>[3x]RRHKNKNPFHFNSKRFQTLFKNQYGHVRVLQRFNKRSQQLQNLRDYRILEFNSKPNTLLLPHHADADYLIVILNGTAILTLVNNDDRDSYNLQSGDALRVPAGTTYYVVNPDNDENLRMITLAIPVNKPGRFESFFLSSTQAQQSYLQGFSKNILEASYDTKFE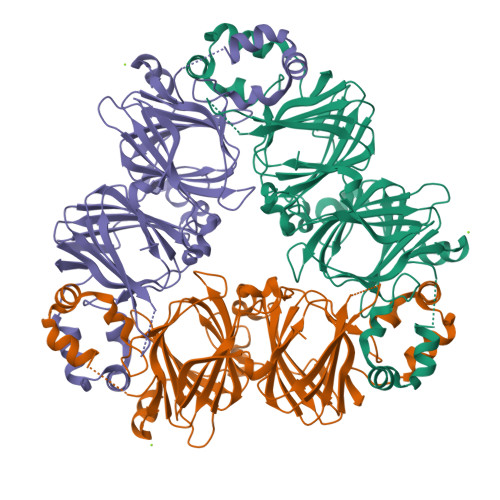EINKVLFGREEGQQQGEERLQESVIVEISKKQIRELSKHAKSSSRKTISSEDKPFNLRSRDPIYSNKLGKLFEITPEKNPQLRDLDVFLSVVDMNEGALFLPHFNSKAIVVLVINEGEANIELVGIKEQQQRQQQEEQPLEVRKYRAELSEQDIFVIPAGYPVVVNATSDLNFFAFGINAENNQRNFLAGSKDNVISQIPSQVQELAFPGSAKDIENLIKSQSESYFVDAQPQQKEEGNKGRKGPLSSILRAFY> SGSSEQELAAIVRDLGCGPYFLGTHDKRFPGFLAGNKLACAIVNTAGRETG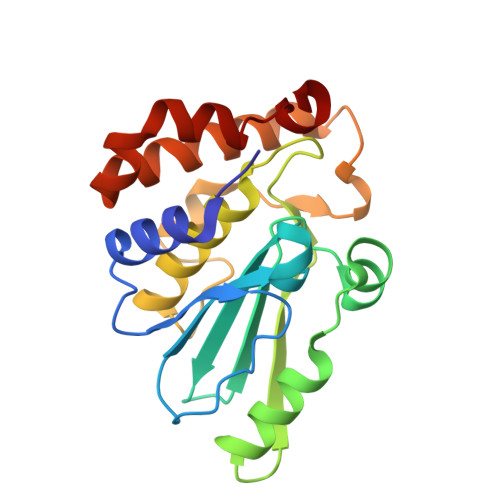GVHWLAFGWNPRSRTCYMFDPFGFSDRRLKQIYSFEYEAMLRRSALALSPDRCLSLEQSTQTVQGPDSAACGLFCCMFLHAFVHWPDRPMDGNPTMNLLTGVPNGMLQSPQVLPTLRRNQEKLYRFLAHHSPYFRSHRAAIEHATAFDKMKQL>[2x]MGSDKIHHHHHHMPKIWTERIFDDPEIYVLRIDDDRIRYFEAVWEIPEGISYNAYLVKLNGANVLIDGWKGNYAKEFIDALSKIVDPKEITHIIVNHTEPDNSGSLPATLKTIGHDVEIIASNFGKRLLEGFYGIKDVTVVKD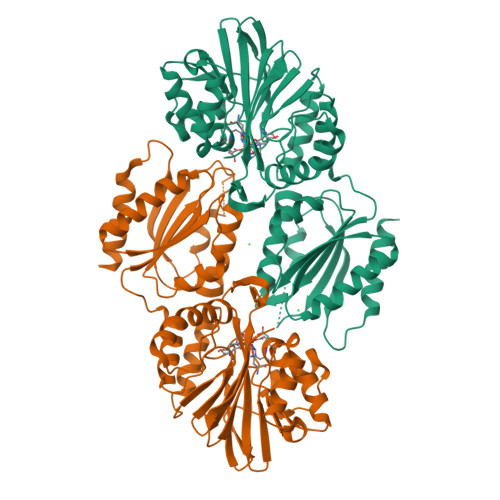GEEREIGGKKFKFVMTPWLHWPDTMVTYLDGILFSCDVGGGYLLPEILDDSNESVVERYLPHVTKYIVTVIGHYKNYILEGAEKLSSLKIKALLPGHGLIWKKDPQRLLNHYVSVAKGDPKKGKVTVIYDSMYGFVENVMKKAIDSLKEKGFTPVVYKFSDEERPAISEILKDIPDSEALIFGVSTYEAEIHPLMRFTLLEIIDKANYEKPVLVFGVHGWAPSAERTAGELLKETKFRILSFTEIKGSNMDERKIEEAISLLKKELE> MFPFGHKGQKIKGTMVVMQ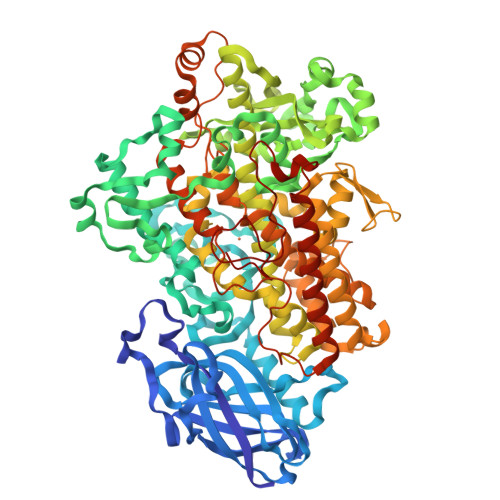KNVLDINSITSVDGIVGTGLDFLGSALDTVTFLASSISIQLISATKADGGKGKVGKATNLRGKITLPTIGAKEEAYDAQFDWDSDFGIPGAFYIKNYMQNEFYLKSLILEDIPNHGTIHFICNSWVYNSKHYKTDRIFFANNTYLPSETPAPLVKYREEELKNVRGDGTGERKEWDRIYDYDVYNDLGDPDKGEKYARPVLGGSALPYPRRGRTGRGKTRKDPNSEKPGDFVYLPRDEAFGHLKSSDFLAYGIKSVAQDVLPVLTDAFDGNLLSLDFDNFAEVRKLYEGGVTLPTNFLSNITPIPIIKELFRTDGEQFLKYPPPKVMQVDKSAWMTDEEFARETIAGLNPNVIKIIEEFPLSSKLDTQAYGDHTCIITKEHLEPNLGGLTVEQAIQNKKLFILDHHDYLIPYLRKINANTTKTYATRTIFFLKNDGTLTPLAIELSKPHPQGEEYGPVSEVYVPSSEGVEAYIWLLAKAYVVVNDACYHQIISHWLNTHAVVEPFVIATNRHLSVVHPIYKLLFPHYRDTMNINSLARKSLVNADGIIEKTFLWGRYSLEMSAVIYKDWVFTDQALPNDLVKRGVAVKDPSAPHGVRLLIEDYPYASDGLEIWDAIKSWVEEYVSFYYKSDEELQKDPELQAWWKELVEVGHGDLKDKPWWQKMQTREELVEASATLIWIASALHAAVNFGQYPYGGLILNRPTISRRFMPEKGSPEYDALAKNPEKEFLKTITGKKETLIDLTIIEILSRHASDEFYLGQRDGGDYWTSDAGPLEAFKRFGKNLEEIEKKLIEKNNDETLRNRYGPAKMPYTLLYPSSEEGLTFRGIPNSISI>[3x]SHMTPDIILQRT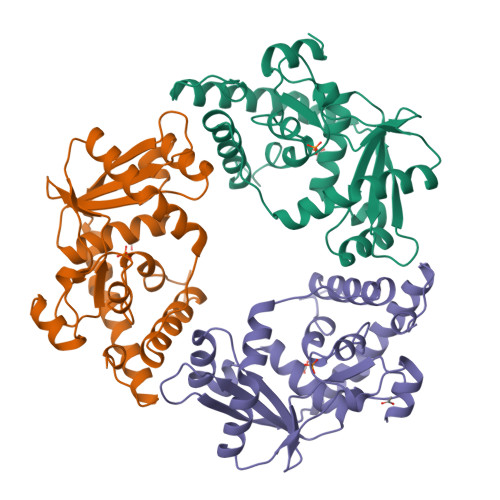GIDVRAVEQGDDAWHKLRLGVITASEVHNVIAKPRSGKKWPDMKMSYFHTLLAEVCTGVAPEVNAKALAWGKQYENDARTLFEFTSGVNVTESPIIYRDESMRTACSPDGLCSDGNGLELKCPFTSRDFMKFRLGGFEAIKSAYMAQVQYSMWVTRKNAWYFANYDPRMKREGLHYVVIERDEKYMASFDEIVPEFIEKMDEALAEIGFVFGEQWR> MMKLKSNQTRTYDGDGYKKRAACLCFRSESEEEVLLVSSSRHPDRWIVPGGGMEPEEEPSVAAVREVCEEAGVKGTLGRLVGIFENQERKHRTYVYVLIVTEVLEDWEDSVNIGRKREWFKIEDAIKVLQYHKPVQASYFETLRQGYS

We have biochemically and structurally characterized a minimalist inositol phosphate kinase (i.e., TvIPK) encoded by Terrestrivirus, a nucleocytoplasmic large (“giant”) DNA virus (NCLDV). We show that TvIPK can synthesize inositol pyrophosphates from a range of scyllo- and myo-IPs, both in vitro and when expressed in yeast cells. We find a heart-shaped ligand binding pocket comprising an array of positively charged and flexible side chains, underlying the observed substrate diversity. A crucial arginine residue in a conserved “G-loop” orients the γ-phosphate of ATP to allow substrate pyrophosphorylation.

To determine structures of TvIPK products, these were purified and soaked into crystals of human DIPP1; this experiment does not exclude the possibility that a substrate yields multiple products, only one of which is captured in DIPP1 crystal complexes. We suggest that minor conformational changes are also required to rotate the plane of the inositol ring by 60° to establish catalytic productivity for two substrate configurations that we have captured in our TvIPK crystal complexes: those for scyllo-IP5 and scyllo-IP6. This proposal is consistent with our demonstration that TvIPK pyrophosphorylates the 3-phosphate of scyllo-IP5 (Figure EV1). In any case, these data provide further validation that TvIPK selectively adds a β-phosphate to pre-existing phosphate, and thus exclusively synthesizes PP-IPs.>[12x]GPELMVISRAEIYWADLGPPSGSQPAKRRPVLVIQSDPYNASRLATVIAAVITSNTALAAMPGNVFLPATTTRLPRDSVVNVTAIVTLNKTDLTDRVGEVPASLMHEVDRGLRRVLDL

MazEF is a TA system implicated in the formation of “persisters cells” of M. tb, which contain more than 10 such members. All the MazF toxins from the family are RNases, capable of cleaving various types of RNA including mRNA, tRNA, or rRNA. To better reflect the specificity of MazF-mt3 in M. tb, the so-called MORE RNA-seq was developed, which identified the cleavage sequence as U↓CCUU. Here we report crystal structures of MazF-mt3 in its apo form and in complex with the C-terminal half of MazE-mt3.

We next crystallized and solved the apo structure of MazF-mt3 at 3.3 Å, using the alphafold 2-predicted structure as the search model for the molecular replacement. The space group is P43212, and the unit cell is rather large, with the three dimensions measuring 110.8, 110.8, and 271.2 Å. There are 12 MazF-mt3 monomers present in the asymmetric unit (ASU), assembling into six dimers. Most chains resolved nearly all the residues except for an internal proline-rich loop of a 9-residue length between β1 and β2. The two monomers were closely associated with each other and were also very similar in structure (a 0.4 Å RMSD over 105 Cαs). Each subunit displays a typical MazF fold, featuring a central antiparallel β-sheet composed of six strands. The helices are mostly short, except for the last helix α3, which also forms part of the dimer interface. The formation of the dimer buries a surface area of 2853.8 Å2. Another notable feature is that α3 in MazF-mt3 is rich in Arg (Arg106, Arg109−110), which forms inter-subunit salt bridges or hydrogen bonds. On the other hand, Arg110′ and Val111′ of α3′ form an intersubunit hydrogen bond with Tyr35 and Ser32, respectively. These interactions contribute to the stabilization of the dimer interface of MazF-mt3 and may be protein-specific because the residues involved are not conserved in the homologs.> MVFYAFVLVMKPRQRRFTSQALREIAVAIYNNGGLIRKLSNEGVMRPYSRFRDADNTPLTYARYVTLQVDMGEEQMRKVEKIMKEHQDVFITLNLNNLERPVGIRRGRKDLQSAYFPLDTFTRLEEE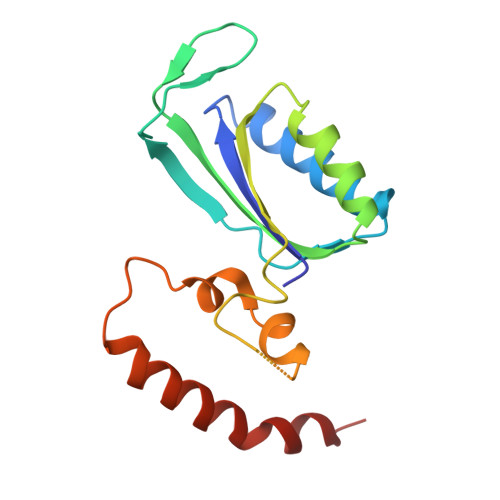INWPPQTSADIYKQLEMNWKEFSRTRWSNFLRN>[2x]MVQYIFTPWRNRAELLAVRAQFYPEHTSKTHLKKHHQSTFQDDEHIRSEKQKAVARVSMWMQRGGCPHMVESTALLVAAILSDEAQGSGAAGGYAVRAAYSAAFSRFVTGLLDSHQDKQRKQSMYDVAKAVGLPAAFVELRHQATHEQLPSLTRLRSAARRALEWIWWYYWKGLGPVDMVQRGVNGKGVAGVGDTSESEEKDVGEEGGDAAARCREGVVRLLESDVRVGGEAINGPGKEELLAEFGEALVLTTLDAAAGNTRDVGVLRRAIGLMREIVNGGDEDCMQLENGKGNRDVEKLKEELKKGWEEIKRLAQEKEDSGDDQTEDEDVDMEAEEEDKKEQQSGWVLYDEKEWVPKPIGIV;>MTSTKKRKLEGSASESGNNTPILSAFAARQQLWAQSLVVQAQKQPQSVDNSKHVTERRSATPISAAQVLRKSKRKSPEDSPITPATPATPVETEEEKPSKPSSPRELLRHHSSFQPNNSNFQRKAGGRLVLSTPDVERFVILGNYGVKVHQGEVTIAGATLTPIDDVQWVHAPHCHALPVLRTANDTVIELLPCPTAQGLRELARLNPLFGRLWNETSDTFQIIYTSADAPKRTSLRELASHPAWNKKISELLTSTRRKPSPILFICGPKSSGKSTFGRLLTNRLMTDRAGHKSRSWKPVMVLDLDPGQPEFSPPGVVSLTKLRRPNLAPPFCHPGLSFGEKGLDGGNEGMTTVRMHAIASVTPALDPAHFIACARDLFAYYRRSASQENIPLVVNTPGWIQGTGLDLLAELIAVLRPTEVLYMSEDGPEETVSALREACASSSTIPFTMLPSQPNSSGEGGGGGAASWTPATLRSMAMQSYFHLSPFSRDQQGGPGCEWNPTPLTHLCPWRVRLAGRPDERGVLGIVCYDHQYAPELVSDAINGMVMGLVRIEKKEALRGLAVPGDTSLSFTSSTSQGGCDDELDSDSNSSSAPSFTSSSPSHLNSTPLLPLIPNPTGSPLSPQYTSLVGLVLIRGVSLTASNPELHLLTPVPPSVLHSFRGDELVLVAGKFDAPTWAYVEGLYWKSNSKAAKRVDEEREDEDREESGGVEEEEEQDEVPWVEMLHGSAGRDVGSRVWRVRRDLGRS[2x]

The rixosome defined in Schizosaccharomyces pombe and humans performs diverse roles in pre‐ribosomal RNA processing and gene silencing. Here, we isolate and describe the conserved rixosome from Chaetomium thermophilum, which consists of two sub‐modules, the sphere‐like Rix1‐Ipi3‐Ipi1 and the butterfly‐like Las1‐Grc3 complex, connected by a flexible linker. The Rix1 complex of the rixosome utilizes Sda1 as landing platform on nucleoplasmic pre‐60S particles to wedge between the 5S rRNA tip and L1‐stalk, thereby facilitating the 180° rotation of the immature 5S RNP towards its mature conformation. Upon rixosome positioning, the other sub‐module with Las1 endonuclease and Grc3 polynucleotide‐kinase can reach a strategic position at the pre‐60S foot to cleave and 5′ phosphorylate the nearby ITS2 pre‐rRNA.

However, wild‐type ct PTF‐Las1 still co‐enriched Las1‐Grc3 together with Rix1‐Ipi1‐Ipi3, but not Rat1‐Rai1, and all five subunits remained stably associated during extended sucrose gradient centrifugation. Since the Rix1‐Ipi3‐Ipi1 complex is known to exhibit a large hollow sphere with a diameter of ~9 nm in yeast (Barrio‐Garcia et al, 2016; Kater et al, 2020) and the reconstituted ct Las1‐Grc3 heterodimer a butterfly‐like structure of 13 nm × 7 nm (Pillon et al, 2017), we conclude that we can observe the entire rixosome by electron microscopy. Once again, we observed the spherical density, which we attribute to the Rix1‐complex, and the butterfly‐shaped Las1‐Grc3, both arranged in such a way that the shorter edge of Las1‐Grc3 is preferentially oriented toward the Rix1 complex, with a distance of about 35 Å. While the cryo‐EM reconstruction of the complete rixosome could only be resolved at low resolution and did not reveal any apparent connecting density, both sub‐complexes could be resolved individually to resolutions of 2.9 Å (Rix1 complex) and 3.0 Å (Las1‐Grc3 complex). Characteristically, the Las1‐Grc3 assembly displayed a two‐fold symmetry as observed previously, with two copies of Las1 and Grc3 and without densities for nucleotides or RNA, thus representing the apo‐state (Pillon et al, 2019). E The Las1‐Grc3 was found in the apo‐state. Strikingly, AF2 multimer predicted with high consistency an interaction between the Las1‐CC and an intertwined bundle of two CC α‐helices formed by the two C‐termini of Ipi3 (Fig EV1B). The Las1‐Grc3 has a high degree of flexibility when attached to the Rix1 complex, but this is probably necessary to fulfill its specific function on the pre‐60S particles, reaching the C2 cleavage site for endonucleolytic cleavage and RNA 5′‐end phosphorylation, which is also in the highly flexible and exposed part of ITS2.>GSRRASVGSHRFKVFNYMSPTFCDHCGSLLWGLVKQGL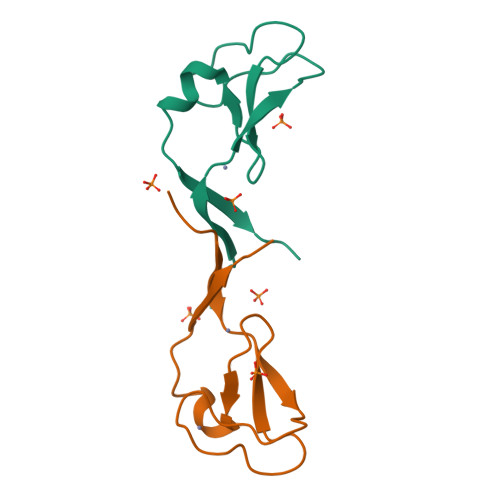KCEDCGMNVHHKCREKVANLCEFIVTD[2x]L-RHAMNITOL | C6 H14 O5 | 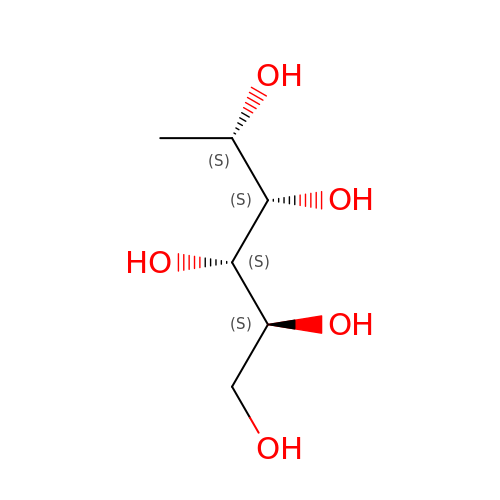SKCKOFZKJLZSFA-BXKVDMCESA-N> MAHHHHHHMKKTSAQKYQESEGDELNYPLGNIDDYSVNNRIGRGKYSNVFSGHIIDSGKPIVVKVLKPVRIMKINREIAILNVLRNGPNISQLLDVVKDPDSKYISLILNYAENNDVKTLFGKMTTRDIALYIYGVLRALAFAHKNGIM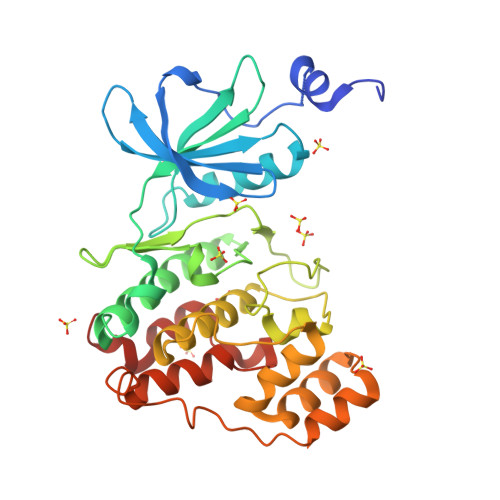HRDVKPGNIMWNQTTKEVSLIDWGLAEFYTPDSEYQVRVATKYYKGPELLLSYLKYTPSLDIWCLGCTLAGLLFHKLPFFKGRDSNEQIERMCVYLGGQAMLDYAEKYDLKLSSSLKARLSELKGTMWAGLINESNRDICTPQALDLLTKMLTIDHNLRPTAEQAMKHPFFDEIRDSVK>PMFIVNTNVPRASVPDGFLSELTQQLAQATGKPPQYIAVHVVPDQLMAFGGSSEPCALCSLGSIG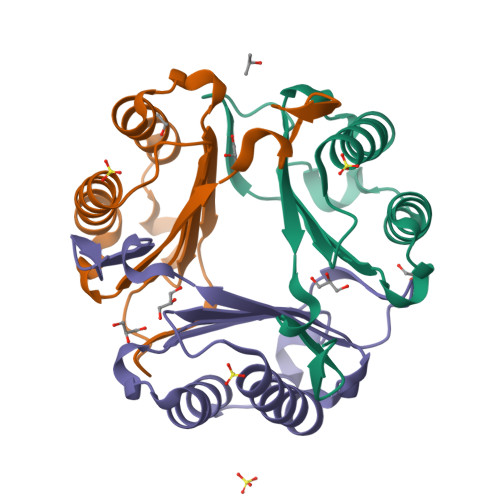KIGGAQNRSYSKLLCGLLAERLRISPDRVYINYYDMNAANVGWNNSTFA[3x]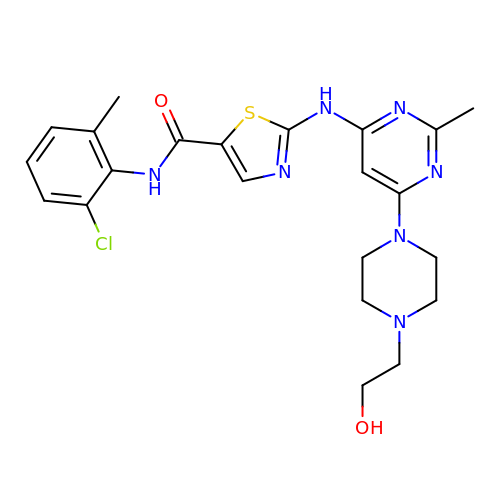N-(2-CHLORO-6-METHYLPHENYL)-2-({6-[4-(2-HYDROXYETHYL)PIPERAZIN-1-YL]-2-METHYLPYRIMIDIN-4-YL}AMINO)-1,3-THIAZOLE-5-CARBOXAMIDE | C22 H26 Cl N7 O2 S | ZBNZXTGUTAYRHI-UHFFFAOYSA-N>MAIILPKLKYALNALSPHISEETLNFHYNKHHAGYVNKLNGLIKDTPFATKSLVEIMKESTGAIFNNAAQIWNHSFYWDSMGPNCGGEPHGEIKEKIQEDFGSFNNFKNEFSNVLCGHFGSGWGWLVLNNNNKLVILQTHDAGNPIKDNTGIPILTCDIWEHAYYIDYRNDRPSYVKAWWNLVNWNFANENLKKAL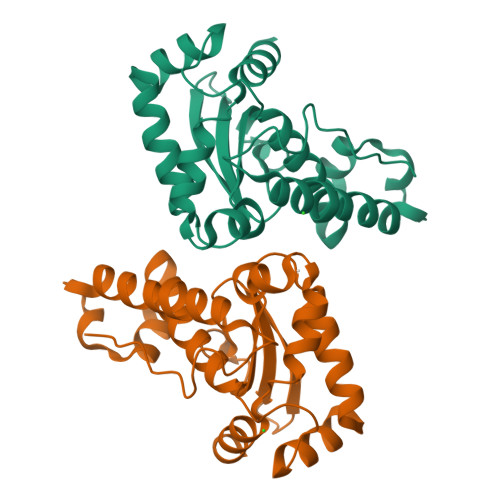QK[2x]>MAFYKREMFDPAEKYKMDHRRRGIALIFNHERFFWHLTLPERRGTCADRDNLTRRFSDLGFEVKCFNDLKAEELLLKIHEVSTVSHADADCFVCVFLSHGEGNHIYAYDAKIEIQ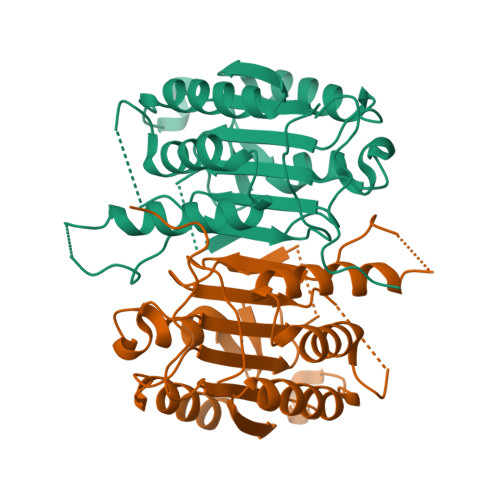TLTGLFKGDKCHSLVGKPKIFIIQACRGNQHDVPVIPLDVVDNQTEKLDTNITEVDAASVYTLPAGADFLMCYSVAEGYYSHRETVNGSWYIQDLCEMLGKYGSSLEFTELLTLVNRKVDQRRVDFCKDPSAIGKKQVPCFASMLTKKLHFFPKSNHHHHHH[8x]> EATAGTVTVNAITSDDTIDGIELGQTISISGKAVGGDISVGDVVKMTINNTEYSTTVKAGGIWMIAGVLGSDLAADSEFDVVVTSSDAAGNKVQSIGTSTHSVDLSAEANFSLAEGQQHVLTNLPEGFGFPDGTTEVVTNFGGTITLGDDGEYRYDAPVRDHGDAVSDKDSVTVTLEDGRTFTVNLDIQDSAPVAVDDQDSIVVQHEEFEVSEIAASWVSYTHGESVTTFDGTSDLGGVDNDSAKDQIRWGNPAESKQSGYGFIDNDSNLEGRFDLNQDISVGTFTHYNYPVYSGGAITSAEMSVEFSVLDHLGVSTPVTLTVNFDHNETPNTNDVNASRDIVTVQNTHVTFERDGDIYTVQIVGFREVGNPDGEVVTSIYTNENAATSYELVVRVVEGDGYSLPSTEGNIFDDNGLGADSLGADGSVTVVGVAVGAIVSSNESVGHSIEGQYGNLVLNSDGSYVYDVTASVSDIPAGATESFAYLIQDQDGSTSSANLSIN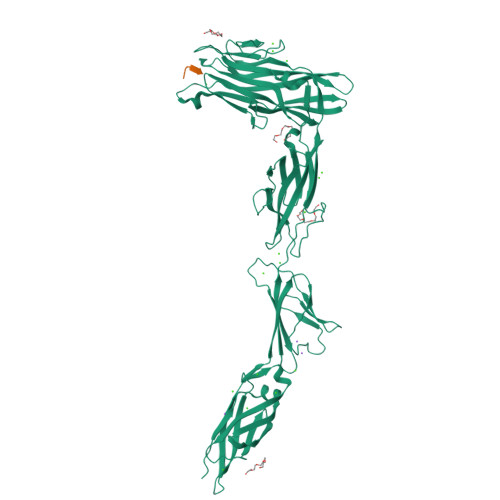VGTN;> AGYTD> CDLNINDDPNYPMNDQVTADLIFPSISASIASAVGGEIYNYAGFFAQYYEQKPESNQYNTLCEYTFTESSQQMDYSYRILFAGALEDAKQVLEKTTNPADRFATTILRAYAFQIMVDNTSDSPYSEALQGNANATPKWDTGETVYKGILGEIDAAEAALDGSGMDVPDLIFNKNIAQWKGFANALRLRMYLRFIDANIDAASYTEKVKTLVQNNEFFTGDVKLDCFLDETDKRNPWYN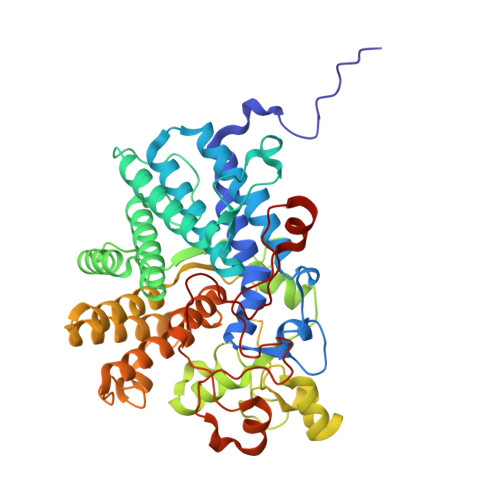TNAVGLTGNHCAAYPLVSYLSSTGDPRIAYGISKTDADGKYVGQLPGGKTHMQSILGTDNWKNKNVSAIDYSIGATKPVYFFTQAELQFLIAEVYARFHNDDANAKSAYEAGVTADFAVRGFAGQENTILEGACAWSAASTQADKLNLIYMQKWVSLFYMDHMEAWSEIRRTDCPKLSSYSAAQIQASESVYTPGELVAPWTNGLEAGGLMKRMTYPLSARQQNVNTPAGVPGSTPVWWDIK>[2x]MREDTKVYDITIIGGGPVGLFTAFYGGMRQASVKIIESLPQLG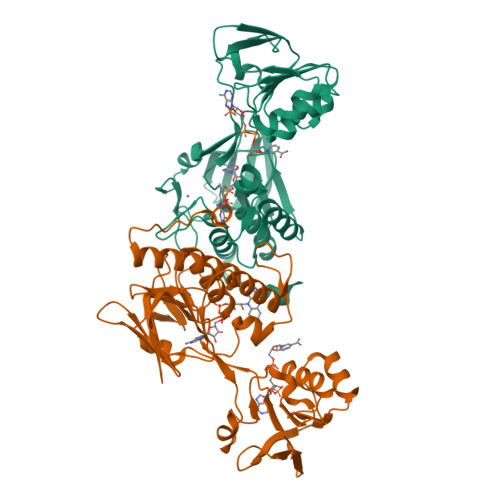GQLSALYPEKYIYDVAGFPKIRAQELINNLKEQMAKFDQTICLEQAVESVEKQADGVFKLVTNEETHYSKTVIITAGNGAFKPRKLELENAEQYEGKNLHYFVDDLQKFAGRRVAILGGGDSAVDWALMLEPIAKEVSIIHRRDKFRAHEHSVENLHASKVNVLTPFVPAELIGEDKIEQLVLEEVKGDRKEILEIDDLIVNYGFVSSLGPIKNWGLDIEKNSIVVKSTMETNIEGFFAAGDICTYEGKVNLIASGFGEAPTAVNNAKAYMDPKARVQPLHSTSLFENK> MSFRYTNNLIGALKHRLLLESSYREIASRKFIGNCRGVEVVCSGYGTVLAVQLTDKAVWESFYRKGGRPTVSGGGDVSGDAETGTQGSATTTGATGSLDLDKLAESIKTALWDATRKIRSAKEAALHRSLSHNTRMRASADLKHWYEEDANT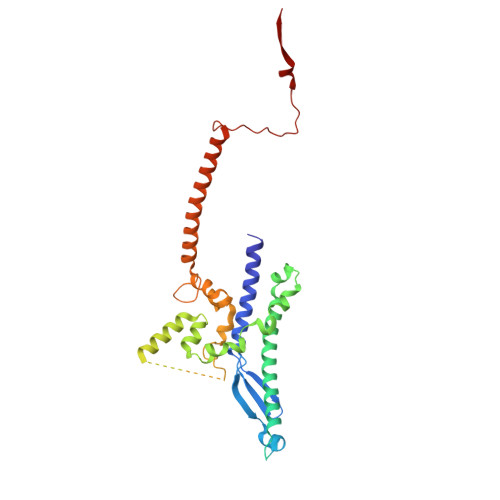LRPLAFEALKHEAATPWMQLVQHGKKEEAAALLKEFEQKGDAAEATPTRVKDDRVKGTRTELSNREQPPLASTLKAEDSNPATIPIGSVHPLFTPALVQIEEAGGGSVSNEAVCRAQLWELSRDEQLFWERVELIRKGQVASIGSSHKRGYADEAAFAKDDTEEKVQLRFTQ NAL catalyses the reversible aldol condensation of N-acetylmannosamine with pyruvate to yield the sialic acid, N-acetylneuraminic acid (Neu5Ac). NAL is a class I aldolase, functioning through the formation of an enzyme–pyruvate Schiff base formed with Lys165 which carries out a nucleophilic attack on the aldehyde carbon of the open-chain form of the N-acetylmannosamine. Here, using the NAL from Staphylococcus aureus, we demonstrate quantitative conversion of a cysteine residue, site-specifically into the nonproteogenic amino acid γ-thialysine, chosen as a mimic of the natural catalytic lysine residue at position 165, using the double alkylation-elimination method and that high yields of an active, modified NAL can be purified. We then characterise the resulting enzyme activity, analyse the pH-dependency of catalysis and use X-ray crystallography to investigate the structural basis of the changes brought about by modifying the enzyme.

The purified protein was shown to have NAL activity and the kinetic parameters determined were similar to those of the E. coli NAL. In the wild-type enzyme the average Cβ–Cγ and Cγ–Cδ bond lengths in Lys165 in the four polypeptide chains in the tetramer are both 1.5 Å and the Cβ–Cγ–Cδ bond angle is 110.1°, in excellent agreement with the values of 1.53 Å, 1.54 Å and 110.0° found in free lysine. The pH profile for the wild-type S. aureus enzyme shows a typical bell-shaped profile with a pH optimum of 7.4 and two pKa values of 5.8 and 8.7.

>[4x]HHHHHHNKDLKGLYAALLVPFDENGQVNEQGLKQIAQNAIETEELDGLYVNGSSGENFLLNTEQKKQVFKVAKEAVGDKVKLIAQVGSLDLNEAIELGKYATELGYDALSAVTPFYYPFTFEEIRDYYFDIIEATQNNMIIYAIPDLTGVNISIEQFSELFNHEKIVGVKYTAPNFFLLERIRKAFPDKLILSGFDEMLVQATISGVDGAIGSTYNVNGRRARKIFDLARQGQIQEAYQLQHDSNDIIETVLSMGIYPTLKEILRHRGIDAGLPKRPFKPFNEAHRQTLDQLIAKYDL> AIADVGTDRYAPYFAYAAAQPSDEVTTVRGLSNPLIKTAPVTLPFDLGQAVADNCLSLSGMGYYLGLGGCCPTCAAAEPRLGRSDRAALVLAYVQQLNSIYEYRVFLASVAARDPSERALEEVLAHPELFFAYYVLRDGGLRDVRVLFFEDPDAQGALMMYVVFPEKSVHVHHRVLDRLLGACAGHRIVAHVWQTMFVLVVRKKGDGRPADDVPAVSASDIYCKMRDISFDGELLLEY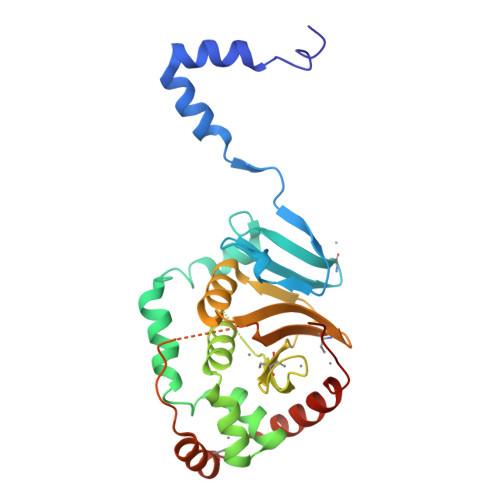KRLYAAFEDFRPPRP> MCRKNRFFALAG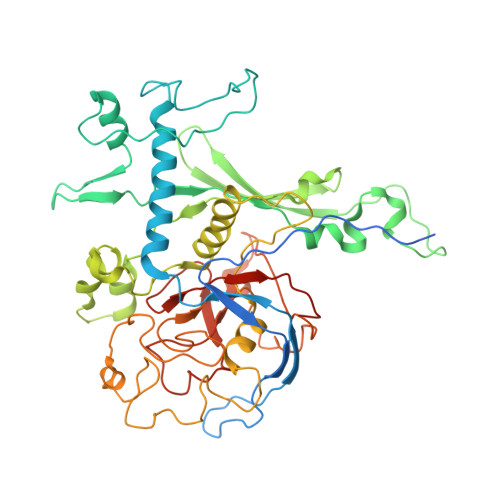FFLFGVFTISSCGSSKRAVGGELTGAKLSSWNEPSPFGMIQVPRGSIVLGNKEADSLWGIPAESRPISVDAFWMDRTEITNAQYRQFVYYVRDSIIRERLADPAYGGNEEYKITENKFGEPVTPHLDWSKPIPSEKRATEEEIAAINSVYYTNPVTHDRKLNPDQMVYRYEVYDYRSAALREHQLKAAKRNLNTDIKVDPNAVVMISKDTAFVDESGNIISETITRPLSSEYDFLNTYIVPIYPDETCWVNDFPNARTEIYTRMYFNHPGYDDYPVVGISWEQAQAFCAWRSEFFRKGIRLPEGQIMDDFRLPTEAEWEYAARMGDSNNKYPWSTEDLRTGRGCFLGNFKPGEGDYTADGHLIPSRVSSFSPNDFGLYDMAGNVAEWTSTAFSESGLKQMSDINPELEYKAALTDPYILKQKVVRGGSWKDVARFIRSATRSHEYQNVGRSYIGFRCVRTSIAFSSGKAPKSSRRSIKK> GSMSLNDFLSSVLPVSEQFEYLSLQSIPLETHAVVTPNKDDKRVPKSTIKTQHFFSLFHQGKVFFSLEVYVYVTLWDEADAERLIFVSKADTNGYCNTRVSVRDITKIILEFILSIDPNYYLQKVKPAIRSYKKISPELISAASTPARTLRILARRLKQSGSTVLKEIESPRFQQDLYLSFTCPREILTKICLFTRPASQYLFPDSSKNSKKHILNGEELMKWWGFILDRLLIECFQNDTQAKLRIPGEDPARVRSYLRGMKYPLWQVGDIFTSKENSLAVYNIPLFPDDPKARFIHQLAEEDRLLKVSLSSFWIELQERQEFKLSVTSSVMGISGYSLATPSLFPSSADVIVPKSRKQFRAIKKYITGEEYDTEEGAIEAFTNIRDFLLLRMATNLQSLTGKREHRERNQPVPASNINTLAITMLKPRKKAKALPKT;> MMSDQENENEHAKAF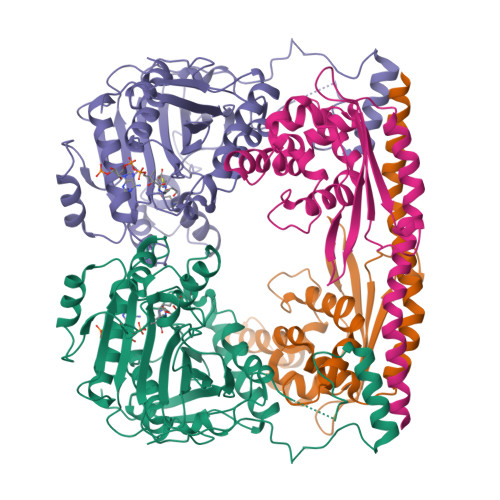LGLAKCEEEVDAIEREVELYRLNKMKPVYEKRDAYIDEIAEFWKIVLSQHVSFANYIRASDFKYIDTIDKIKVEWLALESEMYDTRDFSITFHFHGIEGDFKEQQVTKVFQIKKGKDDQEDGILTSEPVPIEWPQSYDSINPDLIKDKRSPEGKKKYRQGMKTIFGWFRWTGLKPGKEFPHGDSLASLFSEEIYPFCVKYYAEAQRDLEDEEGESGL> ELHIGGIFPIAGKGGWQGGQACMPATRLALDDVNKQPNLLPGFKLILHSNDSECEPGLGASVMYNLLYNKPQKLMLLAGCSTVCTTVAEAAKMWNLIVLCYGASSPALSDRKRFPTLFRTHPSATVHNPTRIKLMKKFGWSRVAILQQAEEVFISTVEDLENR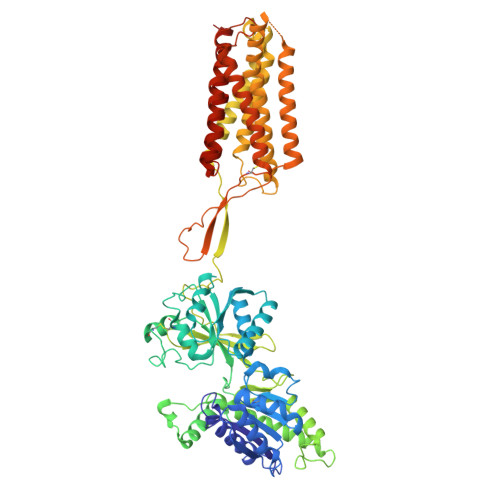CMEAGVEIVTRQSFLSDPTDAVRNLRRQDARIIVGLFYVVAARRVLCEMYKQQLYGRAHVWFFIGWYEDNWYEVNLKAEGITCTVEQMRIAAEGHLTTEALMWNQNNQTTISGMTAEEFRHRLNQALIEEGYDINHDRYPEGYQEAPLAYDAVWSVALAFNKTMERLTTGKKSLRDFTYTDKEIADEIYAAMNSTQFLGVSGVVAFSSQGDRIALTQIEQMIDGKYEKLGYYDTQLDNLSWLNTEQWIGGKVPQDRTIVTHVLRTVSLPLFVCMCTISSCGIFVAFALIIFNIWNKHRRVIQSSHPVCNTIMLFGVIICLISVILLGIDGRFVSPEEYPKICQARAWLLSTGFTLAYGAMFSKVWRVHRFTTKAKTDPKKKVEPWKLYTMVSGLLSIDLVILLSWQIFDPLQRYLETFPLEDPVSTTDDIKIRPELEHCESQRNSMWLGLVYGFKGLILVFGLFLAYETRSIKVKQINDSRYVGMSIYNVVVLCLITAPVGMVIASQQDASFAFVALAVIFCCFLSMLLIFVPKVIEVIRH>MRGSHHHHHHGSMSTTIQYNSNYADYSISSYLREWANNFGDIDQAPAETKDRGSFSGSSTLFSGTQYAIGSSHSNPEGMIAEGDLKASFMPQHTFHGQIDTLQFGKDLATNAGGPSAGKHLEKIDITFNELDLSGEFDSGK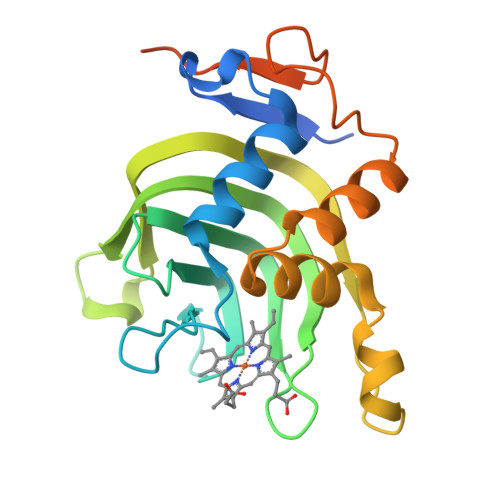SMTENHQGDMHKSVRGLMKGNPDPMLEVMKAKGINVDTAFKDLSIASQYPDSGYMSDAPMVDTVGVMDSNDMLLAA[8x]> 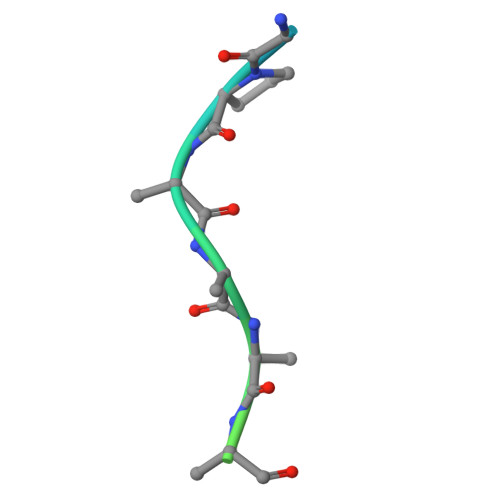GPYEGPVKKPVALKVKAKNLIVTE PYRIDINE-N-OXIDE 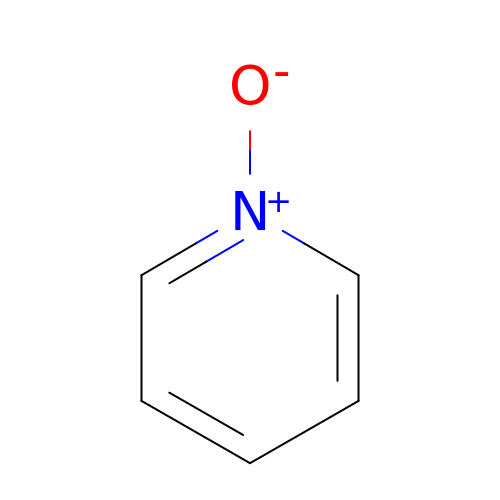| C5 H5 N O | ILVXOBCQQYKLDS-UHFFFAOYSA-N>GSGAMERVLKVFHYFENSSEPTTWASIIRHGDATDVRGIIQKIVDCHKVKNVACYGLRLSHLQSEEVHWLHLDMGVSNVREKFELAHPPEEWKYELRIRYLPKGFLNQFTEDKPTLNFFYQQVKNDYMLEIADQVDQEIALKLGCLEIRRSYGEMRGNALEKKSNYEVLEKDVGLRRFFPKSLLDSVAAATLAALIQQTFRQFANLNREESILKFFEILSPVYRFDKECFKCALGSSWIISVELAIGPEEGISYLTDKGANPTHLADFNQVQTIQYSNSEDKDRKGMLQLKIAGAPEPLTVTAPSLTIAENMADLIDGYCRLVNGATQSFIIRPQKEGERALPSIPKLANNEKQGVRSHTVSVSETDDY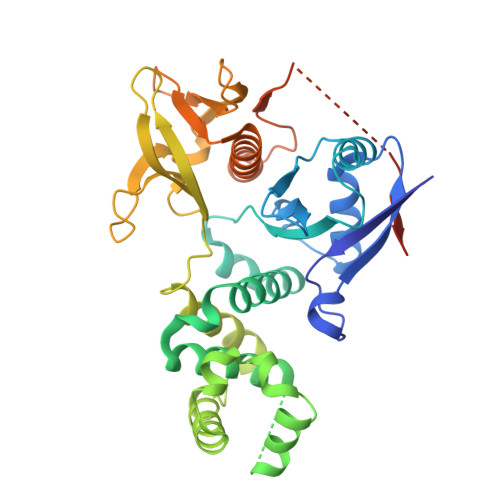AEIIDEED[2x]>[2x]AMNYFVGNSLGVNLTGIEKAIINRLNLFKEMGRPAQCVFLSWNRYLYRNAQNYITSSDYINMYDFFQEATYLERNEPFDWLSYWTDECHYTLKHVENSHDFRIYDQERFLMYAHFQDPKYRILDYVNHFDSQRRKVKRDFYDVRGFLSCSRILVDKQQTLCEFFYNPEGDTKLEKYFSYKDGKPEVQKIIVYYANKQYFFNNETELGAFFIKQLYQHGDLFFSDRNVYTAPIFNLTPESIPVVAVLHSTHIKNIDALDSSPFKNVYKAMFENLSRYRAIIVSTEQQKLDVEKRINHTIPVVNIPVGYSETIDTPVQTLDQRSVKLISVARYSPEKQLHQQIELIKRLVSYVPKIELHMYGFGSESKKLNELIQKYGLENHVYLRGFLSNLDQEYSDAYLSLITSNMEGFSLALLESLAHGVPVISYDIKYGPNELI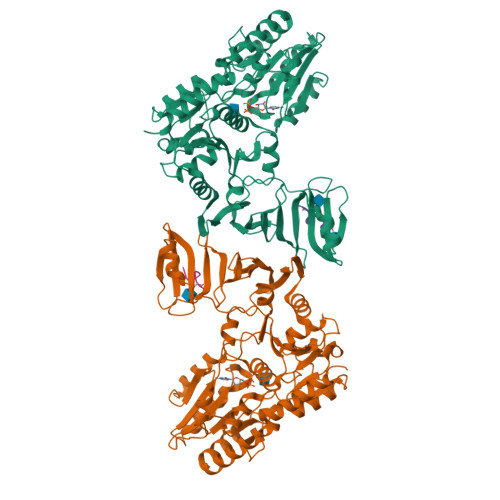TSDFNGYLITKNDEDALFDKVKYVIDHPEVQQRLSKGSLAKAQQYSKASLIKQWDQFVRLILEHHHHHH;>[2x]DSDSDSDSD> DDHSELLVNTKSGKVMGTRVPVLSSHISAFLGIPFAEPPVGNMRFRRPEPKKPWSGVWNASTYPNNCQQYVDEQFPGFSGSEMWNPNREMSEDCLYLNIWVPSPRPKSTTVMVWIYGGGFYSGSSTLDVYNGKYLAYTEEVVLVSLSYRVGAFGFLALHGSQEAPGNVGLLDQRMALQWVHDNIQFFGGDPKTVTIFGESAGGASVGMHILSPGSRDLFRRAILQSGSPNCPWASVSVAEGRRRAVELGRNLNCNLNSDEELIHCLREKKPQELIDVEWNVLPFDSIFRFSFVPVIDGEFFPTSLESMLNSGNFKKTQILLGVNKDEGSFFLLYGAPGFSKDSESKISREDFMSGVKLSVPHANDLGLDAVTLQYTDWMDDNNGIKNRDGLDDIVGDHNVICPLMHFVNKYTKFGNGTYLYFFNHRASNLVWPEWMGVIHGYEIEFVFGLPLVKELNYTAEEEALSRRIMHYWATFAKTGNPNEPHSQESKWPLFTTKEQKFIDLNTEPMKVHQRLRVQMCVFWN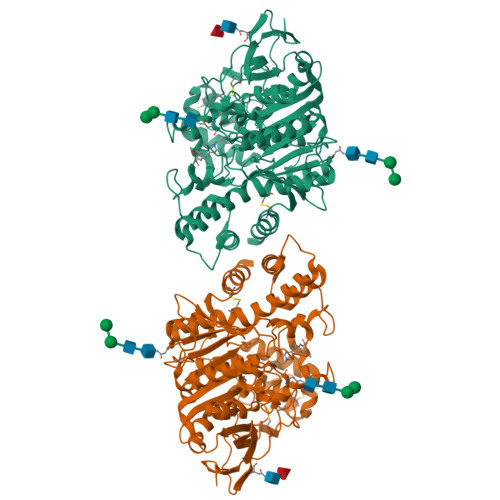QFLPKLLNATACDGELSS> GPLGSGSSIRVKLL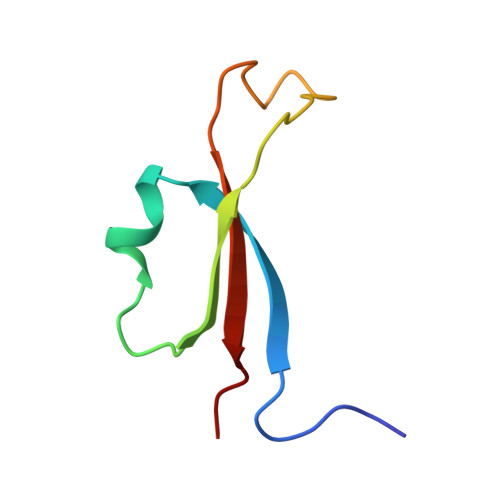QESVVKLNPKLVKHNFYRVEANDSEEEETEFDDQFCIADIQLVD> DQNTEEMENLSDRVASDKAGNSATNTQSTVGRLCGYGKSHHGEHPASCADTATDKVLAAERYYTIDLASWTTSQ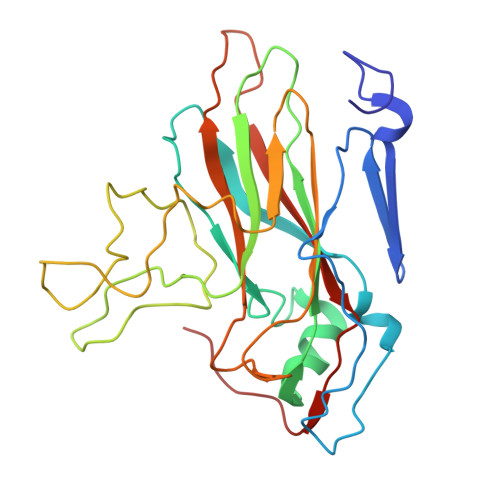EAFSHIRIPLPHVLAGEDGGVFGATLRRHYLCKTGWRVQVQCNASQFHAGSLLVFMAPEFYTGKGTKTGTMEPSDPFTMDTEWRSPQGAPTGYRYDSRTGFFATNHQNQWQWTVYPHQILNLRTNTTVDLEVPYVNVAPSSSWTQHANWTLVVAVLSPLQYATGSSPDVQITASLQPVNPVFNGLRHETVIAQ> MRRLPLFCRRPSRCCGATASGSGSSSAAVLAASAAPSVLVLAARGIATSGRVTNEDRRWWLVHLECAPDVTPGTFVSWLDCCGTHTTKKLIERNIWTIEQVAELDSDRVDELKYKEGCLKMDVVWEHARTIITPLKQREVSGGVESQLQSRILELRKKRELERQRELLARERATVSDKREETLRRLRESVAAKK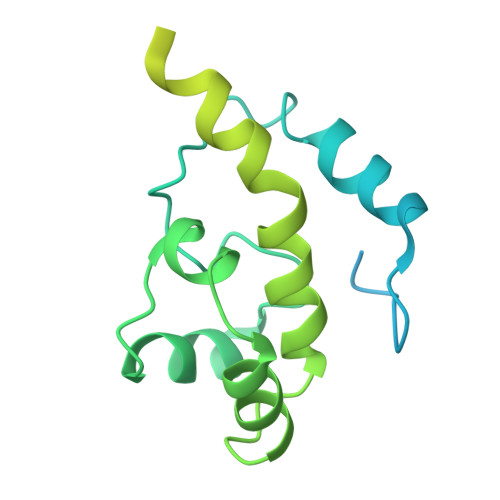AALRKKLDEQHGEATPAASESASTEAHRGTAEAAVEDEAVGNIVDRMSGGNPPRA1H-indazol-6-amine | C7 H7 N3 | 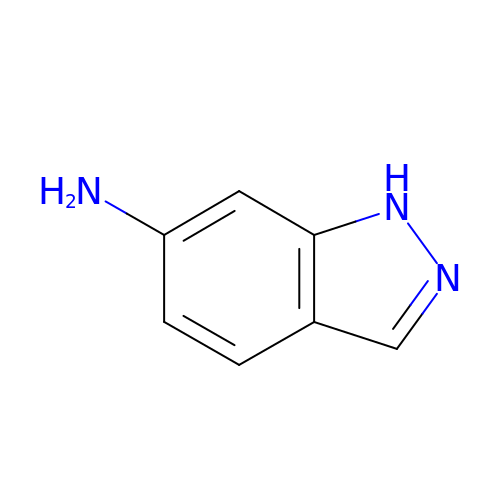KEJFADGISRFLFO-UHFFFAOYSA-N L-xylulose-5-phosphate 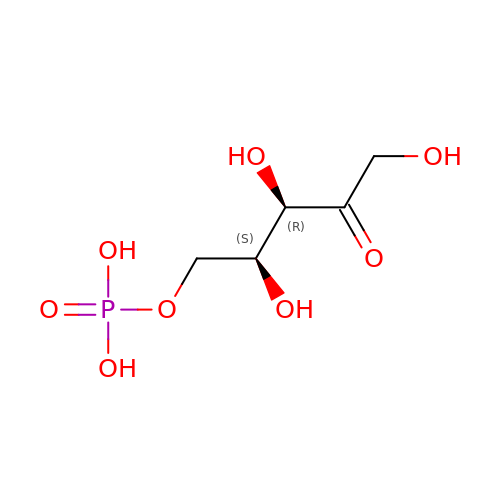| C5 H11 O8 P | FNZLKVNUWIIPSJ-WHFBIAKZSA-N>[2x]MFIRIKCFSKQPIAKKVSREVSAYLEYTGNNTWEGHISGQGVSNLQTKLINVGKGVK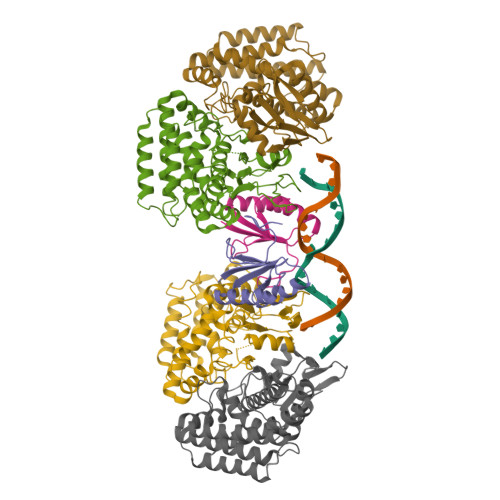VVCNYQDKVLFAIGNVAMSDTGSV;>[4x]MQKQILTSQKRNMYILSRCKVLVKNGQVCHLHEDGNVYTVPYANTVFIGLAEGTSITNEAMSMLAANGVIVFWTKGGGYDMFAADIICHLPQADYRPTKYMQNWVRLWLDEEKKLSAAKEILKMRVDSLSTHVHDFGVDVENKRVSSIVNKFDKGVTQATSFESLLGHEGTFVKSLYKEYALEYEIEFKRDHKSADNYNKFLTLGNYYAYGIARSSLWALGIDNSFPLLHGSTRRGGLVFDVADIIKTSIILPLAFHAADQGMSNTEFKRSCVAYFDKNDILAYLINNIKRLCMEN3-azanyl-5-bromanyl-1-methyl-pyridin-2-one | 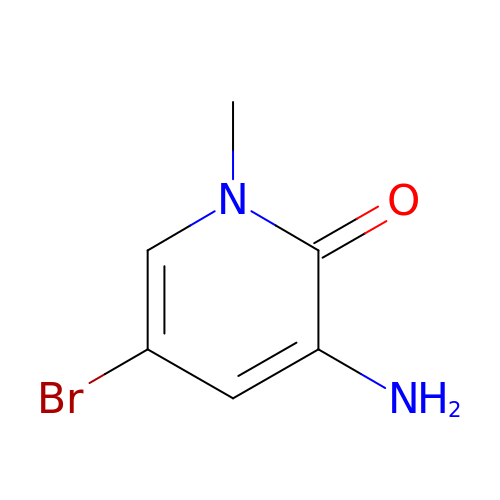C6 H7 Br N2 O | KRUDZWOELKQDJW-UHFFFAOYSA-N> MANPINEFIGIIREEGKYHNQPSFFIGKIKSKLPDLKIETNNIILEKEDILIDSWMIDRQLETFDTETNQEHQHEVKNPFIDNFESGDMVIMFRIGEKFAVVSKLV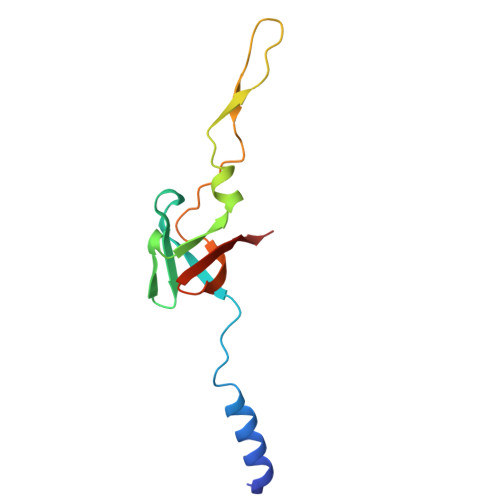SL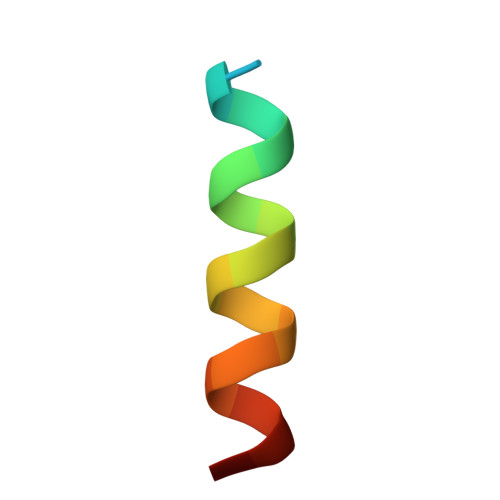> DMRPEIWIAQELRRIGDEFN> MGSN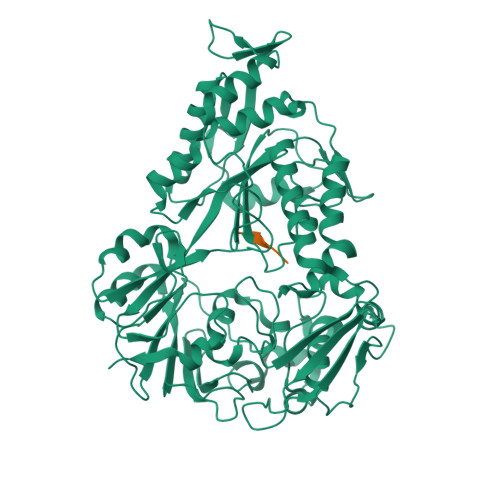QSSSTSTKKLKAGNFDVAYQNPDKAIKGGNLKVAYQSDSPMKAQWLSGLSNDATFATMSGPGGGQDGLFFTDSGFKFIKGGAADVALDKESKTATITLRKDLKWSDGSEVTAKDYEFTYETIANPAYGSDRWTDSLANIVGLSDYHTGKAKTISGITFPDGENGKVIKVQFKEMKPGMTQSGNGYFLETVAPYQYLKDVAPKDLASSPKTTTKPLVTGPFKPENVVAGESIKYVPNPYYWGEKPKLNSITYEVVSTAKSVAALSSSKYDIINGMVSSQYKQVKNLKGYKVLGQQAMYISLMYYNLGHYDAKNSINVQDRKTPLQDQNVRQAIGYARNVAEVDNKFSNGLSTPANSLIPPIFKQFTSSSVKGYEKQDLDKANKLLDEDGWKLNKSTGYREKDGKELSLVYAARVGDANAETIAQNYIQQWKKIGVKVSLYNGKLMEFNSWVDHMTTPPGANDWDITDGSWSLASEPSQQDLFSAAAPYNFGHFNDSEITKDLNDIDSAKSENPTYRKAAFVKYQEDMNKKAYVIPTNFMLNYTPVNKRVVGMTLDYGAMNTWSEIGVSSAKLATKGSIEGRHHHHHH;> SFANG> AYVINDSCIACGACKPECPVNCIQEGSIYAIDADSCIDCGSC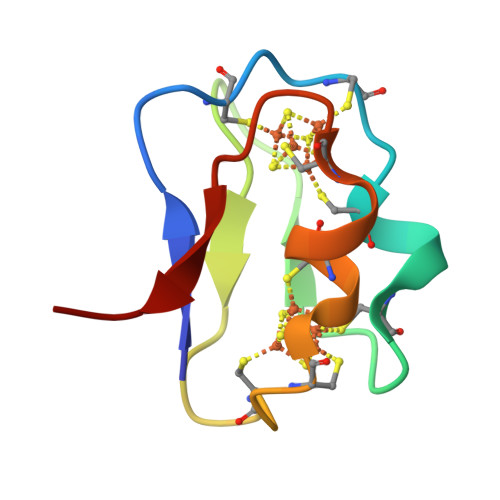ASVCPVGAPNPED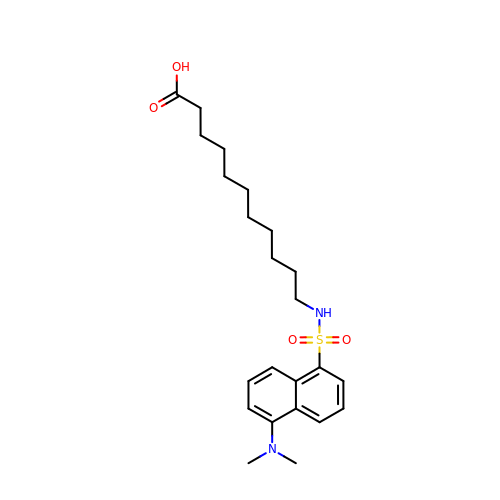11-({[5-(dimethylamino)naphthalen-1-yl]sulfonyl}amino)undecanoic acid | C23 H34 N2 O4 S | CEPGVMDMVJGHFQ-UHFFFAOYSA-N>[3x]KKHSVLHLVPVNITSKADSDVTEVMWQPVLRRGRGLEAQGDIVRVWDTGI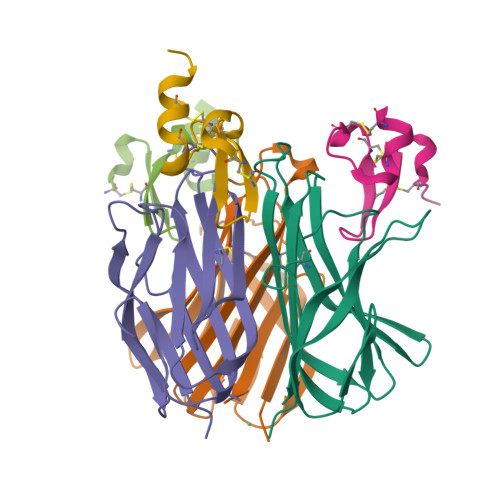YLLYSQVLFHDVTFTMGQVVSREGQGRRETLFRCIRSMPSDPDRAYNSCYSAGVFHLHQGDIITVKIPRANAKLSLSPHGTFLGFVKL;>SLSCRKEQGKFYDHLLRDCISCASICGQHPKQCAYFCENKLR[3x]>MGSSHHHHHHSQDPMSLNLVSEQLLAANGLKHQDLFAILGQLAERRLDYGDLYFQSSYHESWVLEDRIIKDGSYNIDQGVGVRAISGEKTGFAYADQISLLALEQSAQAARTIVRDSGDGKVQTLGAVEHSPLYTSVDPLQSMSREEKLDILRRVDKVAREADKRVQEVTASLSGVYELILVAATDGTLAADVRPLVRLSVSVLVEEDGKRERGASGGGGRFGYEFFLADLDGEVRADAWAKEAVRMALVNLSAVAAPAGTMPVVLGAGWPGVLLHEAVGHGLEGDFNRRGTSVFSGQVGELVASELCTVVDDGTMVDRRGSVAIDDEGTPGQYNVLIENGILKGYMQDKLNARLMGMTPTGNGRRESYAHLPMPRMTNTYMLPGKSTPQEIIESVEYGIYAPNFGGGQVDITSDKFVFSTSEAYLIENGKVTKPVKGATLIGSGIETMQQISMVGNDLKLDNGVGVCGKEGQSLPVGVGQPTLKVDNLTVGGTA[2x];>MALAMKVISQVEAQRKILEEAVSTALELASGKSDGAEVAVSKTTGISVSTRYGEVENVEFNSDGALGITVYHQNRKGSASSTDLSPQAIARTVQAALDIARYTSPDPCAGVADKELLAFDAPDLDLFHPAEVSPDEAIELAARAEQAALQADKRITNTEGGSFNSHYGVKVFGNSHGMLQGYCSTRHSLSSCVIAEENGDMERDYAYTIGRAMSDLQTPEWVGADCARRTLSRLSPRKLSTMKAPVIFANEVATGLFGHLVGAIAGGSVYRKSTFLLDSLGKQILPDWLTIEEHPHLLKGLASTPFDSEGVRTERRDIIKDGILTQWLLTSYSAR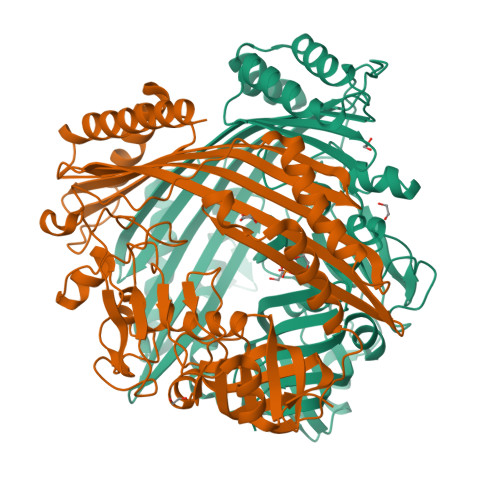KLGLKSTGHAGGIHNWRIAGQGLSFEQMLKEMGTGLVVTELMGQGVSAITGDYSRGAAGFWVENGEIQYPVSEITIAGNLKDMWRNIVTVGNDIETRSNIQCGSVLLPEMKIAGQ[2x]> PSLIHPDTAKYPFKFEPFLRQEYSFSLDPDRPICEFYNSREGPKSCPRGPLCPKKHVLPIFQNKIVCRHWLRGLCK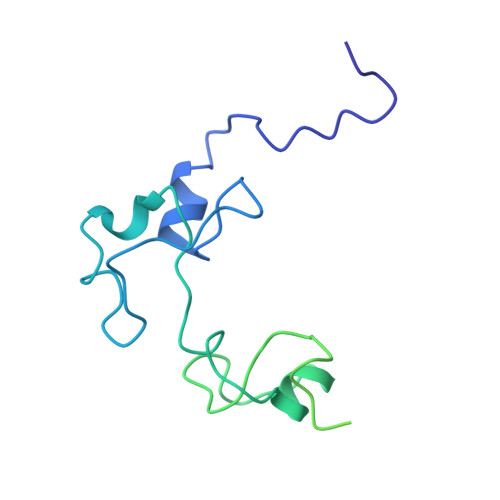KNDQCEYLHEYNLRKMPECVFFSKNGYCTQSPDCQYLHIDPASKIPKCENYEMGFCPLGSSCPRRHIKKVFCQRYMTGFCPLGKDECDMEHPQFIIPDEGSKLRIKRDDEINTRKMDEEKERRLNAIINGEV>[6x]MLQSLNHLTLAVSDLQKSVTFWHELLGLTLHARWNTGAYLTC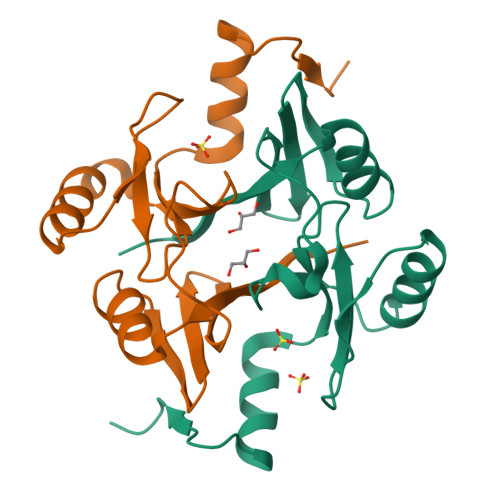GDLWVCLSYDEARQYVPPQESDYTHYAFTVAEEDFEPLSQRLEQAGVTIWKQNKSEGASFYFLDPDGHKLELHVGSLAARLAACREKPYAGMVFTSDEA> AKMAFTLADRVTEEMLADKAALVVEVVEENY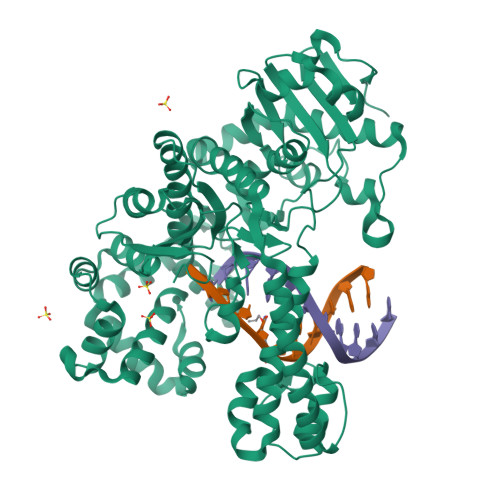HDAPIVGIAVVNEHGRFFLRPETALADPQFVAWLGDETKKKSMFDSKRAAVALKWKGIELCGVSFDLLLAAYLLDPAQGVDDVAAAAKMKQYEAVRPDEAVYGKGAKRAVPDEPVLAEHLVRKAAAIWALERPFLDELRRNEQDRLLVELEQPLSSILAEMEFAGVKVDTKRLEQMGEELAEQLRTVEQRIYELAGQEFNINSPKQLGVILFEKLQLPVLKKSKTGYSTSADVLEKLAPYHEIVENILHYRQLGKLQSTYIEGLLKVVRPDTKKVHTIFNQALTQTGRLSSTEPNLQNIPIRLEEGRKIRQAFVPSESDWLIFAADYSQIELRVLAHIAEDDNLMEAFRRDLDIHTKTAMDIFQVSEDEVTPNMRRQAKAVNFGIVYGISDYGLAQNLNISRKEAAEFIERYFESFPGVKRYMENIVQEAKQKGYVTTLLHRRRYLPDITSRNFNVRSFAERMAMNTPIQGSAADIIKKAMIDLNARLKEERLQARLLLQVHDELILEAPKEEMERLCRLVPEVMEQAVTLRVPLKVDYHYGSTWYDAK>[2x]GPHMEDRAAQSLLNKLIRSNLVDNTNQVEVLQRDPNSPLYSVKSFEELRLKPQLLQGVYAMGFNRPSKIQENALPLMLAEPPQNLIAQSQSGTGKTAAFVLAMLSQVEPANKYPQCLCLSPTYELALQTGKVIEQMGKFYPELKLAYAVRGNKLERGQKISEQIVIGTPGTVLDWCSKLKFIDPKKIKVFVLDEADVMIATQGHQDQSIRIQRMLPRNCQMLLFSATFEDSVWKFAQKVVPDPNVIKLKREEETLDTIKQYYVLCSSRDEKFQALCNLYGAITIAQAMIFCHTRKTASWLAAELSKEGHQVALLSGEMMVEQRAAVIERFREGKEKVLVTTNVCARGIDVEQVSVVINFDLPVDKDGNPDNETYLHRIGRTGRFGKRGLAVNMVDSKHSMNILNRIQEHFNKKIERLDTDDLDEIEKIAN

At the cytoplasmic face of the NPC, Nxf1•Nxt1-bound mRNPs encounter the cytoplasmic filament nucleoporins Gle1, Nup42, and Nup214, which specifically activate the DEAD-box helicase DDX19 to remove Nxf1•Nxt1 from the mRNP8. DDX19 is a member of the DEAD-box helicase family, which are RNA-dependent ATPases composed of two RecA domains (referred to as DDX19NTD and DDX19CTD throughout the text). Gle1CTD plays an important organizational role by providing spatially separated binding sites for Nup42GBM and the DEAD-box helicase DDX19/scDbp5. A comprehensive structure-function analysis of DDX19 indicates that binding of Gle1CTD•Nup42GBM induces a conformational change in DDX19, thereby stimulating its ATPase activity.

Therefore, we used a construct of DDX19 that contained the N-terminal auto-inhibitory helix but did not contain the flexible N-terminal extension (DDX19∆N53, residues 54–479). In addition, we determined the crystal structure of apo DDX19∆N53(AMP-PNP•Mg2+) at 2.2 Å resolution. The surprising observation that AMP-PNP-bound DDX19 could also adopt the auto-inhibited conformation was confirmed by the structure of apo DDX19∆N53(AMP-PNP•Mg2+), which adopted an identical conformation as apo DDX19∆N53(ADP). The inhibited state does not differ structurally in the presence of ADP or ATP, as the nucleotide-binding pocket readily accommodates the additional phosphate and Mg2+ ion, with minor changes in the sidechain conformations of K64 from the auto-inhibitory helix and E243 in the nucleotide binding pocket. DDX19 is predominantly trapped in the auto-inhibited state, which can form in the presence of either ATP or ADP, although the ATP- and ADP-bound states could exhibit different dynamics for release of the auto-inhibitory helix. To gain further insight into how Gle1CTD•Nup42GBM binding facilitates DDX19 activation, we compared the structures of Gle1CTD•Nup42GBM•DDX19∆N53 to those of apo DDX19∆N53. The most apparent difference was a rotation of both DDX19NTD and the auto-inhibitory helix away from DDX19CTD, despite the auto-inhibitory helix still being bound between the two domains.>[5x]GSHMGGVEVLEVKTGVDSITEVECFLTPEMGDPDEHLRGFSKSISISDTFESDSPNRDMLPCYSVARIPLPNLNEDLTCGNILMWEAVTLKTEVIGVTSLMNVHSNGQATHDNGAGKPVQGTSFHFFSVGGEALELQGVLFNYRTKYPDGTIFPKNATVQSQVMNTEHKAYLDKNKAYPVECWVPDPTRNENTRYFGTLTGGENVPPVLHITNTATTVLLDEFGVGPLCKGDNLYLSAVDVCGMFTNRS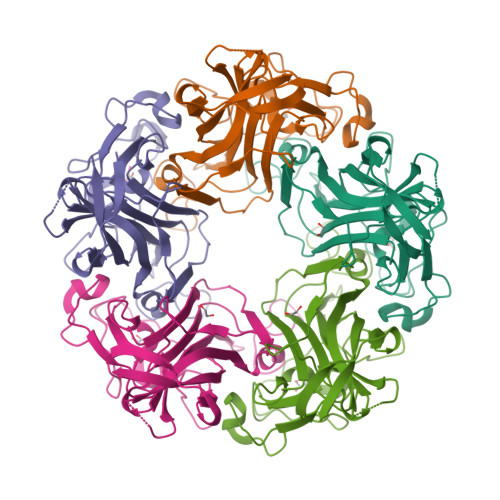GYQQWRGLSRYFKVQLRKRRVKN>[2x]GSHMLSEELRQIVFRTIESLPEDLRMAITLRELDGLSYEEIAAIMDCPVGTVRSRIFRAREAIDNKVQPLIRR

The largest and most diverse subgroup of alternative σ factors, the group IV extracytoplasmic function σ factors, directs the transcription of genes that regulate a wide variety of responses, including envelope stress and pathogenesis. The Ec ECF σ factor σE is an essential protein that directs the response to periplasmic stress. The σE is then free to bind RNAP and drive the transcription of a core set of genes conserved across most bacteria, as well as a more variable set of genes. Promoter-specific transcription initiation first requires the formation of a closed complex in which σ domains 2 (σ2) and 4 (σ4) bind sequence-specifically to the −10 and −35 promoter DNA elements, respectively.

Thin rectangular crystals grown using a 12-bp DNA fragment diffracted to 2.3 Å-resolution. The crystallographically related DNA helices packed head-to-tail, forming a pseudo-continuous double helix with the 1 bp overhangs forming Hoogstein base pairs with the adjacent double helices. Protein–DNA interactions, which occur exclusively within the major groove, extend from −29 to −36, spanning the entire −35 element as well as one base of upstream DNA. Interestingly, the primary base-specific protein–DNA interactions occur at only three positions of the 7-bp −35 element (all Guanines), −35, −34, and −31′. The upstream edge of the −35 element is recognized through a series of hydrogen bonds and van der Waals interactions, mostly between R176 and S172 and the guanine bases at −35 and −34. In addition, R176 forms a cation–π interaction with the −36 DNA base, creating a stair motif along with the −35 hydrogen bonds. The protein–DNA base-specific interactions at the −31′ position are almost exclusively from R171, which makes two hydrogen bonds and one van der Waals interaction with the −31′G. In contrast to the numerous base-specific interactions at the −35, −34, and −31′ positions, the −33 and −32 positions each contain only one base-specific contact, in the form of van der Waals interactions between the thymidine C5-methyl groups at −33′ and −32′ with F175 and R171, respectively. Despite not being a true oligo(dA) • oligo(dT) tract as a result of the cytosine insertion at −31, the σE −35 element DNA is relatively straight, with a high degree of propeller twist, and the minor groove width begins to narrow at the start of the −33/−32 AA. The narrow minor groove is stabilized by a network of cross-strand hydrogen bonds between adjacent DNA bases, along with a spine of hydration consisting of water-mediated hydrogen bonds between the two strands.> HMERPESELIRQSWRVVSRSPLEHGTVLFARLFALEPSLLPLFQGGGQFSSPEDSLSSPEFLDHIRKVMLVIDAAVTNVEDLSSLEEYLTSLGRKHRAVGVRLSSFSTVGES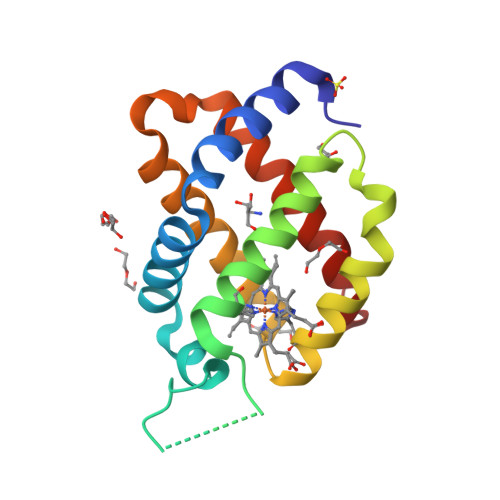LLYMLEKSLGPDFTPATRTAWSRLYGAVVQAMSRGWDGE>GSSPGPYIVRLLNSSLNGCEFPLLTGRTLFVVGQSDALTASGQLPDIPADSFFIPLDHGGVNFEIQVDTDATEIILHELKEGNSESRSVQLNTPIQVGELLILIRPESEPW[6x]

The bacterial injectisome, or type III secretion system (T3SS), is a specialized syringe-shaped protein-export system utilized by many pathogenic Gram-negative bacteria for the injection of virulence proteins (effectors) into host cells. The injectisome can be divided into three major regions: the inner- (IM) and outer-membrane (OM) spanning basal body with associated export apparatus and ATPase components, an extracellular needle, and a terminating pore inserted into the host cell membrane called the translocon. The major structural scaffold of the basal body is comprised largely of three proteins that arrange into a series of highly oligomerized, concentric rings: two intimately associated proteins localized to the IM - PrgK/EscJ/MxiJ and PrgH/EscD/MxiG, and a third protein belonging to the secretin family of OM proteins, InvG/EscC/MxiD (Salmonella enterica serovar Typhimurium SPI-1, Enteropathogenic Escherichia coli (EPEC) LEE and Shigella dysenteriae nomenclature, respectively). In summary, we report the crystal structures for the cytoplasmic and periplasmic domains of PrgH and InvG, two of the main basal body components of the prototypical Salmonella SPI-1 injectisome.

A ∼20° subunit rotation in the hexamer of the crystal structure accommodates the tighter packing but superposition of the interface secondary structural units shows significant conservation with both interfaces having similar buried surface areas (640 Å2 vs. 546 Å2 for hexamer and 24mer respectively). Collectively, the crystallographic packing interfaces we observe support and mirror the low energy interfaces generated in our modelled basal body. This would be consistent with a model whereby the soluble domains have low-affinity interaction surfaces for oligomerization, which can be captured by the high concentration in the crystallization experiment. FHA domains are frequently involved in interaction with phosphothreonine (pThr)-modified proteins. In Shigella, the PrgH orthologue MxiG was reported to interact with phosphorylated peptides from the secretion apparatus protein Spa33 although a separate study failed to corroborate these results, and structures of the Yersinia orthologue YscD revealed an unconserved phosphothreonine binding motif. Protein sequence alignment of the PrgH orthologues indeed illustrates that the conserved residues involved in phosphopeptide binding in FHA domains are poorly conserved. To validate this, we engineered mutations of the PrgH residues corresponding to the proposed phosphothreonine interacting residues in MxiG - Arg35, Gln42 and Asp65 - to alanine. These mutations have no effect on in vivo secretion assays. We therefore conclude that the PrgH cytoplasmic domain is unlikely to interact with pThr-modified proteins. We note however that the FHA phosphopeptide interacting loops in our PrgH structure are accessible on the cytoplasmic face of the ring model, suggesting a potential interface for protein-protein interactions.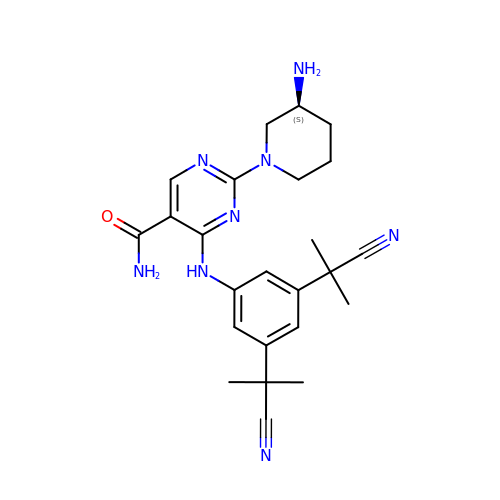2-[(3~{S})-3-azanylpiperidin-1-yl]-4-[[3,5-bis(2-cyanopropan-2-yl)phenyl]amino]pyrimidine-5-carboxamide | C24 H30 N8 O | RJTDRNOTQRMDCY-KRWDZBQOSA-N> MGSSHHHHHHSSGTAEPEVRAKPYTLEEFSYDYFRPPPKHTLSRVMVSKARGKDRLWSHTREPLKQALLKKLLGSEELSQEACLAFIAVLKYMGDYPSKRTRSVNELTDQIFEGPLKAEPLKDEAYVQILKQLTDNHIRYSEERGWELLWLCTGLFPPSNILLPHVQRFLQSRKHCPLAIDCLQRLQKALRNGSRKYPPHLVEVEAIQHKTTQIFHKVYFPDDTDEAFEVESSTKAKDFCQNIATRLLLKSSEGFSLFVKIADKVLSVPENDFFFDFVRHLTDWIKKARPIKDGIVPSLTYQVFFMKKLWTTTVPGKDPMADSIFHYYQELPKYLRGYHKCTREEVLQLGALIYRVKFEEDKSYFPSIPKLLRELVPQDLIRQVSPDDWKRSIVAYFNKHAGKSKEEAKLAFLKLIFKWPTFGSAFFEVKQTTEPNFPEILLIAINKYGVSLIDPKTKDILTTHPFTKISNWSSGNTYFHITIGNLVRGSKLLCETSLGYKMDDLLTSYISQMLTAMSKQRGSRSGK;> GAMGSQDFRKYEEGF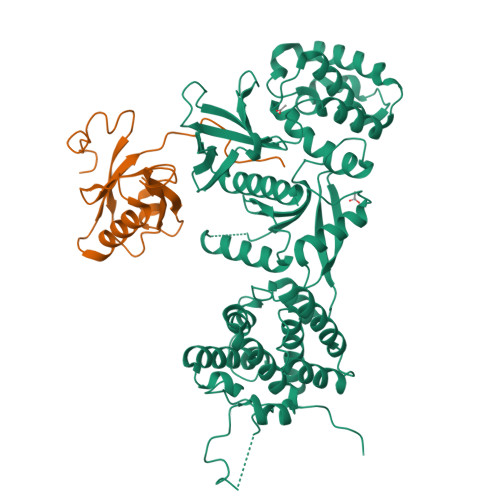DPYSMFTPEQIMGKDVRLLRIKKEGSLDLALEGGVDSPIGKVVVSAVYERGAAERHGGIVKGDEIMAINGKIVTDYTLAEADAALQKAWNQGGDWIDLVVAVCPPKEYDDELTFF>[2x]GSSSRECSYCGKFFRSNYYLNIHLR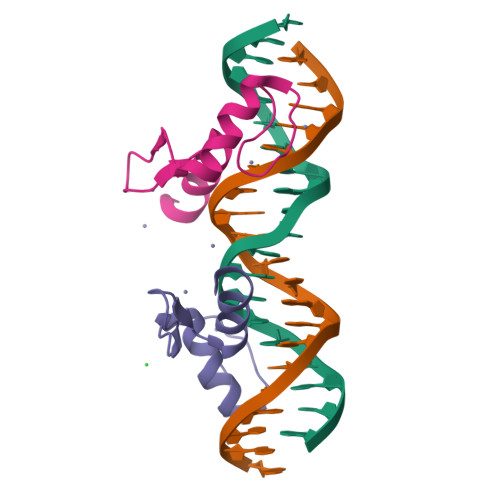THTGEKPYKCEFCEYAAAQKTSLRYHLERHHK>GPLGSSHQQMKASSRRTISQNKRRYRKDGFDLDLTYVTDHVIAMSFPSSGRQSLFRNPIGEVSRFFKTKHPDKFRIYNLCSERGYDETKFDNHVYRVMIDDHNVPTLVDLLKFIDDAKVWMTSDPDHVIAIHCKGGKGRTGTLVSSWLLEDGKFDTAKEALEYFGSRRTDFEVGDVFQGVETASQIRYVGYFEKIKKN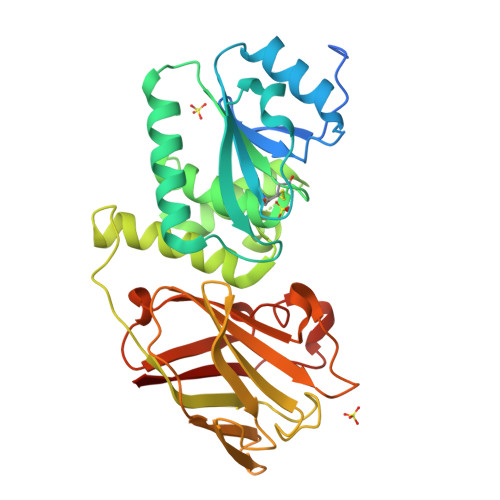YGGQLPPMKKLKVTGVTITAIQGVGRGNGSDLSMQIVSERQEVLLCKFAEGYNCALQYDATDDCVTCEVKNCPVLAGDIKVRFMSTSKSLPRGYDNCPFYFWFNTSLVEGDHVTLKREEIDNPHKKKTWKIYRDNFTVKLTFSDAEDI[3x]>[2x]MEEVVIAGMSGKLPESENLEEFWANLIGGVDMVTADDRRWKAGLYGLPRRMGKLKDLSRFDASFFGVHSKQANTMDPQLRMLLEVTYEAIVDGGINPASLRGTSTGVWVGVSSSDASEALSRDPETLVGYSMIGCQRAMMANRLSFFFDFKGPSITIDTACSSSLLALQSAYQAIRGGECSAAVVGGLNVLLKPNSSLQFMKLGMLSQDGTCRSFDAEGTGYCRAEAVVAVLLTKKSLARRVYATILNAGTNTDGSKEQGVTFPSGDVQEQLIRSLYAPAGPDPESLEYIEAHGTGTKVGDPQELNGIVNALCATRREPLLIGSTKSNMGHPEPASGVAALIKVLLSLEHGVWAPNLHYHTPNPEIPALQDGRLQVVDRPLPIRGGNVGINSFGFGGSNVHVILQPNSRPAPPPAQHAALPRLLQASGRTLEAVQTLLEQGLRHSRDLAFVGMLNEIAAVSPVAMPFRGYAVLGGEAGSQEVQQVPGSKRPVWFICSGMGAQWQGMGLSLMRLDRFRDSILRSDQALKPLGLRVSDLLLSTDEAVLDDIVSSFVSLTSIQIALIDLLTSLGLQPDGIIGHSLGEVACGYADGCLTQEEAVLSSYWRGYCIKEANVLPGAMAAVGLSWEECKQRCPPGIVPACHNSKDTVTISGPQAAMSEFLQQLKREDVFVKEVRTGGIAFHSYFMESIAPTLLRQLRKVILDPKPRSKRWLSTSIPEAQWQGSLARTFSAEYSVNNLVSPVLFQEALQHVPAHAVVVEI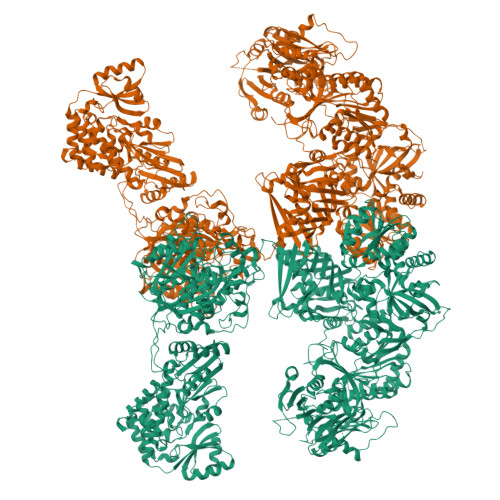APHALLQAVLKRSLESSCTIIPLMKKDHRDNLEFFLSNVGRLHLAGVSVNPNGLFPPVEFPAPRGTPLISPHIKWDHSQAWDVPSAADFPSGSSCSSVAVYKFDVSPESPDHYLVDHCIDGRVLFPGTGYLWLTWKTLARALSQNLEETPVVFEDVTLHQATILPKTGTVSLEVRLLEASHAFEVSDSNGSLIASGKVYQWESPDPKLFDTRAAVDPADSTAEFRLSQGDVYKDLRLRGYDYGPFFQLVLESDLEGNRGRLQWNDSWVSFLDAMLHMSILAPGQLGLYLPTRFTSIRIDPVTHRQKLYTLQDTTQAADVVVDRNLNTVVAGGALFLGAHSSVAPRRPQEHLKPILEKFCFTPHVESGCLAGNTALQEELQLCRGLAQALQTKVAQQGLKMVVPGLDGAQAPREAPQQSLPRLLAAACQLQLNGNLQLELGQVLAQERPLLCDDPLLSGLLDAPALKACVDTALENMASPKMKVVEVLAGDGQLYSRIPALLNTQPVMDLDYTATDRNPQALEAAQAKLEQLHVTQGQWDPANPAPGSLGKADLLVCNCALATLGDPAVAVGNMAATLKEGGFLLLHTLLAGHPLGEMVGFLTSPEQGGRHLLSQDQWESLFAGASLHLVALKRSFYGSVLFLCRQQTPQDSPVFLSVEDTSFRWVDSLKDILADASSRPVWLMAVGCSTSGVVGMVNCLRKEPGGHRIRCVLVSNLSSTSPAPEMHPSSSELQKVLQGDLVMNVYRDGAWGAFRHFPLEQDRPEKQTEHAFVNVLSRGDLSSIRWVCSPLHYALPASCQDRLCSVYYTSLNFRDVMLATGKLSPDSIPGKWLTRDCMLGMEFSGRDASGRRVMGMVPAEGLATSVLLLQHATWEVPSTWTLEEAASVPIVYTTAYYSLVVRGRMQPGESVLIHSGSGGVGQAAIAIALSRGCRVFTTVGSAEKRAYLQARFPQLDETCFANSRDTSFEQHVLRHTAGKGVDLVLNSLAEEKLQASVRCLAQHGRFLEIGKFDLSNNHALGMAVFLKNVTFHGILLDSLFEEGGATWQEVSELLKAGIQEGVVQPLKCTVFPRTKVEAAFRYMAQGKHIGKVVIQVREEEQGPAPRGLPPIALTGLSKTFCPPHKSYVITGGLGGFGLQLAQWLRLRGAQKLVLTSRSGIRTGYQARQVREWRRQGVQVLVSTSNASSLDGARSLITEATQLGPVGGVFNLAMVLRDAVLENQTPEFFQDVSKPKYSGTANLDRVTREACPELDYFVIFSSVSCGRGNAGQANYGFANSAMERICEKRRHDGLPGLAVQWGAIGDVGVVLETMGTNDTVIGGTLPQRIASCLEVLDLFLSQPHPVLSSFVLAEKKAAAPRDGSSQKDLVKAVAHILGIRDVASINPDSTLVDLGLDSLMGVEVRQILEREHDLVLSMREVRQLSLRKLQELSSKTSTDADPATPTSHEDSPVRQQATLNLSTLLVNPEGPTLTRLNSVQSAERPLFLVHPIEGSITVFHGLAAKLSIPTYGLQCTGAAPLDSIQSLASYYIECIRQVQPEGPYRIAGYSYGACVAFEMCSQLQAQQSATPGNHSLFLFDGSHTFVLAYTQSVRAKMTPGCEAEAEAKAMYFFVQQFTDMEQGKVLEALIPLQGLEARVAATVDLITQSHAGLDRHALSFAARSFYQKLRAAENYWPQATYHGNVTLLRAKTGGAYGEDLGADYNLSQVCDGKVSVHVIEGDHRTLLEGSGLESILSIIHSCLAEPRVSVREG>[2x]MAHHHHHHMTEGKKVTIKIGINGFGRIGRMVFRAAQHRNDIEIVGINDLLDADYMAYMLKYDSTHGRYGGMVEVREGALVVNGKKIRVTSERDPANLKWNEVGAVVVVESTGLFLTDETARKHIQAGAKKVVMTGPPKDDTPMFVMGVNNTMYKGQEIVSNASCTTNCLAPLAKIIHEKFGIVEGLMTTVHATTATQKTVDGPSQKDWRGGRGAAQNIIPSATGAAKAVGKVIPALNGRLTGMAFRVP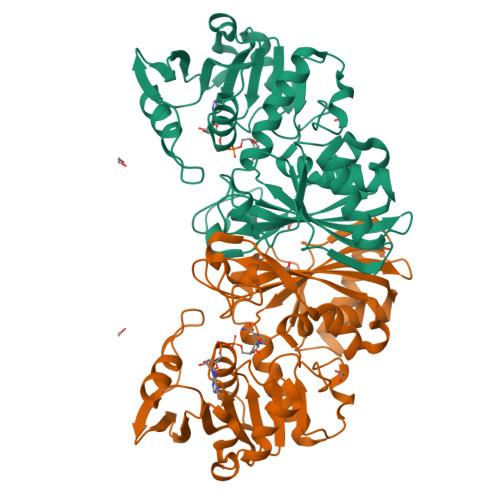TPNVSVVDLTARLERPATYEQICAAIKAASEGELKGILGYTEDEVVSTDMNGVALTSVFDVKAGISLNDRFVKLISWYDNETGYSHKVLDLVAYISAH>[6x]MKAYHIHVQGIVQAVGFRPFVYRIAHEHNLRGYVKNLGDAGVEIVVEGREEDIEAFIEDLYKKKPPLARIDRIEKKEIPPQGFDRFYIEKSSKGGKGGDSIIPPDIAICDDCLRELFDPTNKRYMYPFIVCTNCGPRFTIIEDLPYDRENTTMKEFPMCDFCRSEYEDPLNRRYHAEPTACPVCGPSYRLYTSDGQEIYGDPLRKAAELIDKGYIVAIKGIGGIHLACDAANEEVVAELRRRTFRPQKPFAIMAKDIETVKSFAYVSPEEEEELTSYRRPIITLRKKEPFPLPENLAPGLHTIGVMLPYAGTHYILFHWSKTPVYVMTSANYPGMPMVKDNERAFEELKDVADYFLLHNRKILNRADDSVIRFVDGKRAVIRRSRGFVP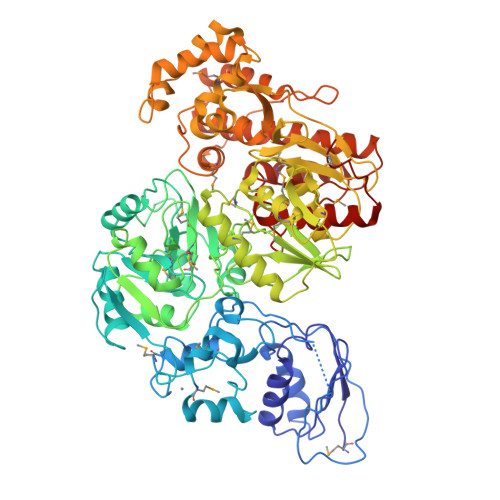LPIEIPFEYNGLAVGAELMNAFGVAKNGKVYPSQYIGNTGKVEVLEFMREAIAHFRKILRVKNLDLIIADLHPAYNTTKLAMEMANELDVELLQVQHHYAHIASVMAEKNLDSVIGIALDGVGYGTDGNTWGGEVLYLGYEDVERLAHIDYYPLPGGDLASYYPLRALMGILSKVYSIDELEGVINRCCPKAVESLKYGKVEFNVVLNQLAKGINTAYASSTGRVLDAIAVLLNVAYRRHYEGEPAMKLESFAFKGKNDLKFEVPVEGELIRVEELFQSILEAIEGASPADIAYSAHLALARAFAHTAVERAREFGVKNVALSGGVAYNELITKMIRKVVEANGLNFHVTTEVPRGDNGVNVGQAFLGGLYLEGYLTKEDLML(3S)-3-({[(5S)-2-{2-[(1H-benzimidazol-5-ylcarbonyl)amino]ethyl}-7-(cyclohexylmethyl)-1,3-dioxo-2,3,5,8-tetrahydro-1H-[1,2,4]triazolo[1,2-a]pyridazin-5-yl]carbonyl}amino)-4-oxopentanoic acid | C29 H35 N7 O7 | 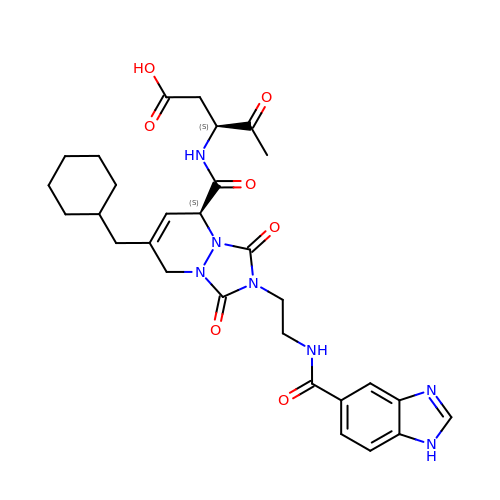CSBIJWXSABAIKK-UPVQGACJSA-N> SRKTYTLTDYLKNTYRLKLYSLRWISDHEYLYKQENNILVFNAEYGNSSVFLENSTFDEFGHSINDYSISPDGQFILLEYNYVKQWRHSYTASYDIYDLNKRQLITEERIPNNTQWVTWSPVGHKLAYVWNNDIYVKIEPNLPSYRITWTGKEDIIYNGITDWVYEEEVFSAYSALWWSPNGTFLAYAQFNDTEVPLIEYSFYSDESLQYPKTV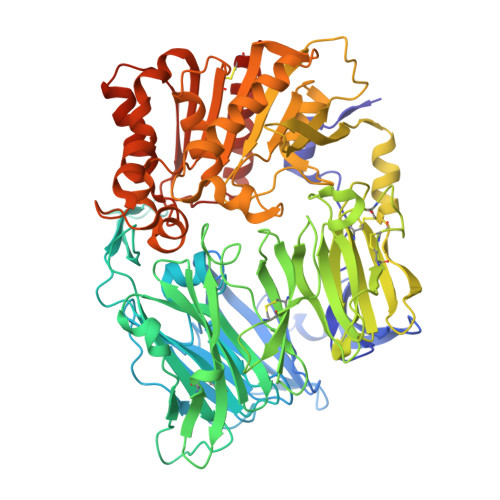RVPYPKAGAVNPTVKFFVVNTDSLSSVTNATSIQITAPASMLIGDHYLCDVTWATQERISLQWLRRIQNYSVMDICDYDESSGRWNCLVARQHIEMSTTGWVGRFRPSEPHFTLDGNSFYKIISNEEGYRHICYFQIDKKDCTFITKGTWEVIGIEALTSDYLYYISNEYKGMPGGRNLYKIQLSDYTKVTCLSCELNPERCQYYSVSFSKEAKYYQLRCSGPGLPLYTLHSSVNDKGLRVLEDNSALDKMLQNVQMPSKKLDFIILNETKFWYQMILPPHFDKSKKYPLLLDVYAGPCSQKADTVFRLNWATYLASTENIIVASFDGRGSGYQGDKIMHAINRRLGTFEVEDQIEAARQFSKMGFVDNKRIAIWGWSYGGYVTSMVLGSGSGVFKCGIAVAPVSRWEYYDSVYTERYMGLPTPEDNLDHYRNSTVMSRAENFKQVEYLLIHGTADDNVHFQQSAQISKALVDVGVDFQAMWYTDEDHGIASSTAHQHIYTHMSHFIKQCFSLPHHHHHH>[2x]GPTTA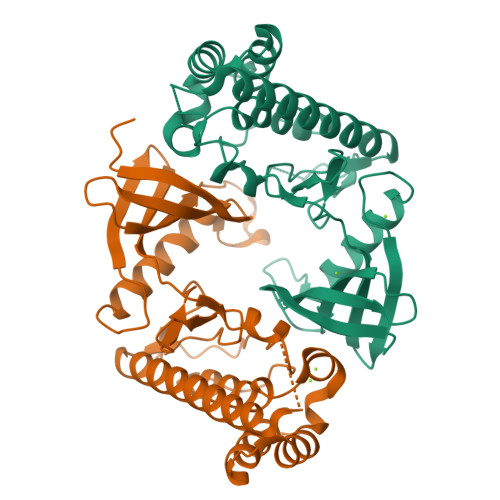GLPYRIEAALHFSNGGGVYAGIDTRTGAQVVLKEARPHAGLAADGADAVTRLRHERDMLQRLAGIDGVPAVLDHFTLGEHHFLVLERIEGRALNTFFAERHPLLDPEPDPGKIADYTAWALRVHAGVERLIDAIHARGIVYNDLHMFNIMVRPDETVALIDFEAAAPLAERSRQTLANPAFQAPPGRYGADVDRYSLACLRLALFLPLTTLLVQDRHKAWELAEAIAEHFPVPRGFLREAAREITRDLPPRPASAAPRFTPDEPGWLQA>MPEIITPIITPFTKDNRIDKEKLKIHAENLIRKGIDKLFVNGTTGLGPSLSPEEKLENLKAVYDVTNKIIFQVGGLNLDDAIRLAKLSKDFDIVGIASYAPYYYPRMSEKHLVKYFKTLCEVSPHPVYLYNYPTATGKDIDAKVAKEIGCFTGVKDTIENIIHTLDYKRLNPNMLVYSGSDMLIATVASTGLDGNVAAGSNYLPEVTVTIKKLAMERKIDEALKLQFLHDEVIEASRIFGSLSSN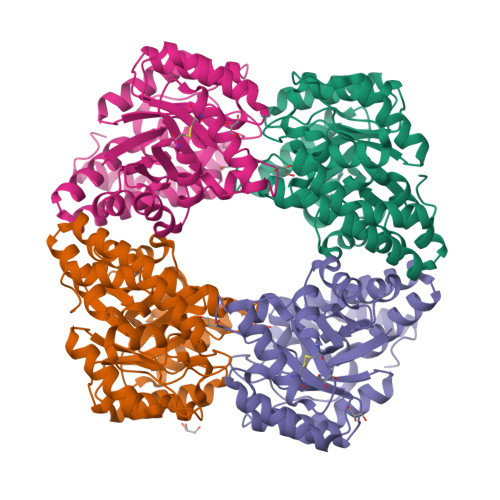YVLTKYFQGYDLGYPRPPIFPLDDEEERQLIKKVEGIRAKLVELKILKE[4x]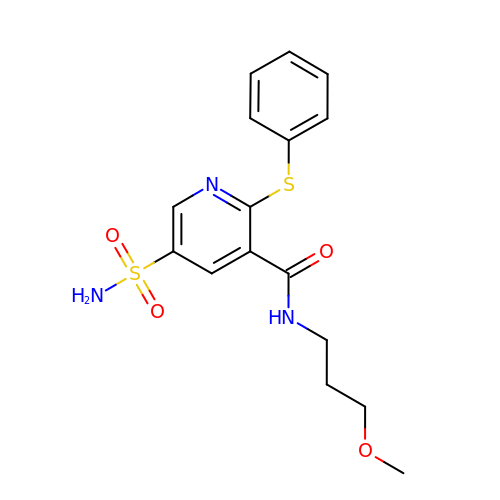N-(3-methoxypropyl)-2-(phenylsulfanyl)-5-sulfamoylpyridine-3-carboxamide | C16 H19 N3 O4 S2 | YFGZGDDAWQULRR-UHFFFAOYSA-N>[5x]MSPGPQSGGQERGSMERKMVELEDTGLTFATEVDLERLQALAAEWLQVIGEDPGREGLLKTPERVAKAWAFLTRGYRQRLEEVVGGAVFPAEGSEMVVVKGVEFYSM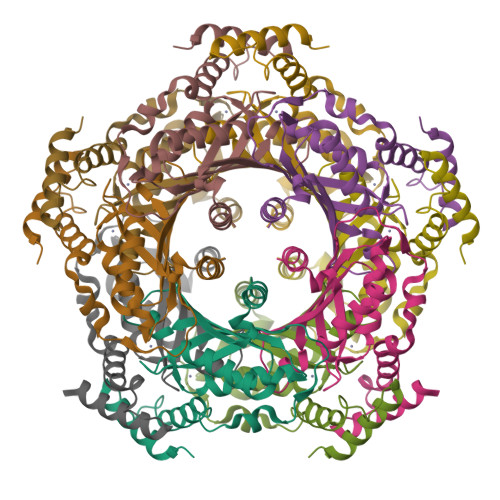CEHHLLPFFGKVHIGYIPDGKILGLSKFARIVDMFARRLQVQERLAVQIAEAIQEVLEPQGVGVVVEGVHLCMMMRGVEKQHSRTVTSAMLGVFRENQKTREEFLSHLRDGTA> MKSVLILAGLVAVALSSAVPKPSTIKTKNVDAVFVEKQKKILSFFQDVSQLNTDDEYYKIGKDYDIEMNMDNYTNKKAVEEFLKMYRTGFMPKNLEFSVFY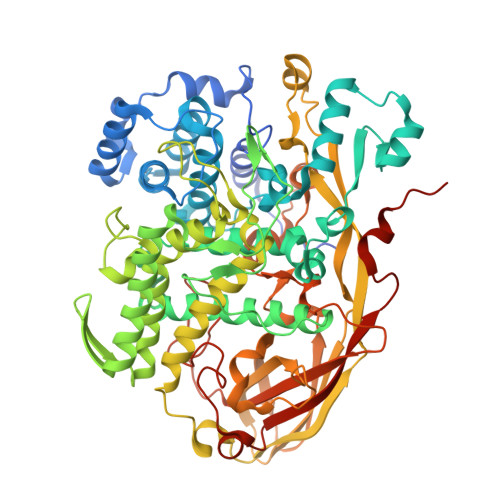DKMRDEAIALFHLFYYAKDFETFYKTACFARVHLNQGQFLYAFYIAVIQRSDCHGFVVPAPYEVYPKMFMNMEVLQKIYVTKMQDGLINPEAAAKYGIHKENDYFVYKANYSNAVLYNNEEQRLTYFTEDIGMNAYYYYFHSHLPFWWTSEKYGALKERRGEVYFYFYQQLLARYYFERLTNGLGKIPEFSWYSPIKTGYYPLMLTKFTPFAQRPDYYNLHTEENYERVRFLDTYEKTFVQFLQKDHFEAFGQKIDFHDPKAINFVGNYWQDNADLYGEEVTKDYQRSYEVFARRVLGAAPMPFDKYTFMPSAMDFYQTSLRDPAFYQLYNRIVEYIVEFKQYLKPYTQDKLYFDGVKITDVKVDKLTTFFENFEFDASNSVYFSKEEIKNNHVHDVKVRQPRLNHSPFNVNIEVDSNVASDAVVKIFLAPKYDDNGIPLTLEDNWMKFFELDWFTTKLTAGQNKIIRNSNEFVIFKEDSVPMTEIMKMLDEGKVPFDMSEEFCYMPKRLMLPRGTEGGFPFQLFVFVYPFDNKGKDLAPFESFVLDNKPLGFPLDRPVVDALFKVPNMYFKDIFIYHEGERFPYKFNIPSYDTQSNVVPKN>[4x]NEALDDIDRIL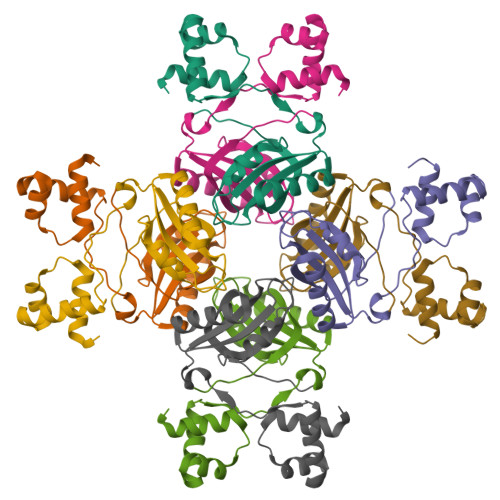VRELAADGRVTLSELATRAGLSVSAVQSRVRRLESRGVVQGYSARINPEAVGHLLSAFVAITPLDPSQPDDAPARLEHIEEVESCYSVAGEESYVMLVRVASARALEDLLQRIRTTANVRTRSTIILNTFYSDRQHIP Fcho1 and Fcho2 likely play a key role in local AP-2 restructuring, as they are among the earliest proteins to mark a nascent CCS (Henne et al., 2010, Taylor et al., 2011) and affect AP-2 conformation directly (Hollopeter et al., 2014, Umasankar et al., 2014). But what makes Fchos unusual is that the C-terminal SH3 domain typical of most EFC-domain proteins is replaced by a μ-homology domain (μHD), distantly related in primary sequence to cargo-selective μ subunits of the heterotetrameric clathrin adaptors such as AP-2 (Reider et al., 2009). The μHD of all three (designated the muniscins) binds directly to the pioneer protein Eps15 (Henne et al., 2010, Reider et al., 2009, Uezu et al., 2007, Umasankar et al., 2012). The structure of an Eps15/R⋅Fcho1 μ-homology domain complex reveals a spacing-dependent DPF triad, bound in a mechanistically distinct way from the mode of single DPF binding to AP-2.

A fusion of EPS15 (designated ET615-EG637) to the zebrafish Fcho1 μHD (residues 867–1,152) with a GAGA spacer crystallized and diffracted to 2.4 Å. In the final structure, excellent-quality electron density is visible for residues EF620-EG637 of EPS15 and P874-L1152 of the μHD. There is no evidence of the spacer residues separating the EPS15 and μHD sections, but distance constraints make it highly likely that the interaction is intramolecular. Like other μ subunits, the Fcho1 μHD contains 18 β strands arranged as two intercalated β-sandwich subdomains, the fold being comparable with the orthologous Saccharomyces cerevisiae Syp1p μHD (Reider et al., 2009) and μ1–μ4. Yet the Fcho1 μHD also contains three additional α helices in subdomain A, and the concave face of the Fcho1 μHD is considerably more curved than other μHDs. The EPS15 segment binds in a spiral trough that runs halfway around the long axis of subdomain A, with the Fcho μHD-unique α helices forming a considerable part of the trough. The trough is lined with conserved largely hydrophobic residues, and significant contacts with the protein are only through the three DPF motif side chains of the sequence 623DPFVGSDPFKDDPF; the interaction buries 1,640 Å2 of solvent-accessible area. The electron density indicates well-ordered DPFs; the first two adopt type I tight turn conformations stabilized by intramolecular H bonding between the Asp residue side chains and the backbone amide of the +2-position Phe residues. In the last DPF, the side chain of ED634 additionally forms a salt bridge with R1133. Thus the structure strongly suggests that the short tri- (VGS) or di- (KD) residue spacing between tandem DPFs is important to allow three to simultaneously dock onto a single Fcho1 subdomain A with a 1:1 stoichiometry.

>[2x]GLSRGPSPISLSAQESWPVAAAITEYINAYFRGGEHNRCLVKITGDLTMSFPAGITRIFTANPNAPVLSFRLVNISRVDHFLPNQKLLYSDPSQSDPDTKDFWFNMQALTLHLQREAELNPQASYYNVALLKYQASSQDPSRAPLLLSAECQRSGTVTRVSLDYHCCPATAPATQLTSVQVLLPLDHSATDLQCQPPAAWNAEERRLLWKLANLSPTNHSKGSGTLCASWQCLEVPRGPAPSLAVQFVGSGASLSGLDVELVGSRYRMSLVKKRFATGKYMAGCSL;>TNLDFFQSDPFVGSDPFKDDPFGGAGA[2x]>SSQRSVARMDGDVIIGALFSVHHQPPAEKVPERKCGEIREQYGIQRVEAMFHTLDKINADPVLLPNITLGSEIRDSCWHSSVALEQSIEFIRDSLISIRDEKDGLNRCLPDGQTLPPGRTKKPIAGVIGPGSSSVAIQVQNLLQLFDIPQIAYSATSIDLSDKTLYKYFLRVVPSDTLQARAMLDIVKRYNWTYVSAVHTEGNYGESGMDAFKELAAQEGLCIAHSDKIYSNAGEKSFDRLLRKLRERLPKARVV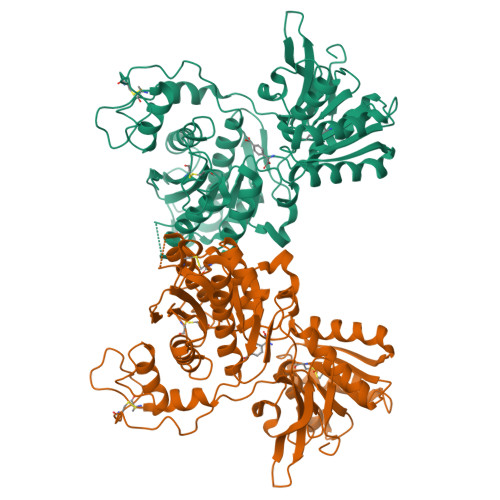VCFCEGMTVRGLLSAMRRLGVVGEFSLIGSDGWADRDEVIEGYEVEANGGITIKLQSPEVRSFDDYFLKLRLDTNTRNPWFPEFWQHRFQCRLPGHLLENPNFKKVCTGNESLEENYVQDSKMGFVINAIYAMAHGLQNMHHALCPGHVGLCDAMKPIDGRKLLDFLIKSSFVGVSGEEVWFDEKGDAPGRYDIMNLQYTEANRYDYVHVGTWHEGVLNIDDYKIQMNKSGMVRS[2x]2-[(2-{(2S,4S)-2-[(R)-(5-tert-butyl-1,3,4-oxadiazol-2-yl)(hydroxy)methyl]-4-fluoropyrrolidin-1-yl}-2-oxoethyl)amino]-2-methylpropan-1-ol | C17 H29 F N4 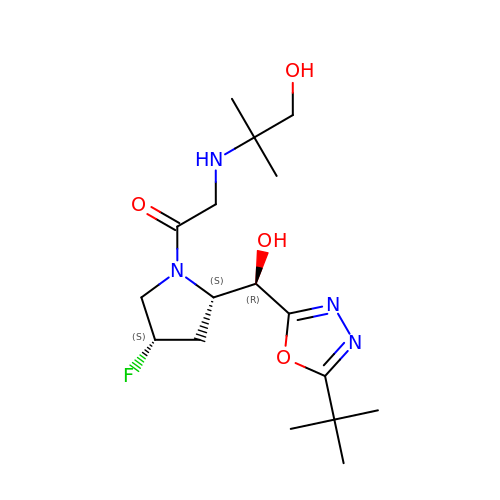O4 | PHTMASAWZAGGEK-GMXVVIOVSA-N> HHHHHHHSSENLYFQGHMRKIRVGLIFGGKSAEHEVSLQSARNILDALDPQRFEPVLIGIDKQGQWHVNDPDSFLLHADDPARIALHRSGRGVALLPGAQQQQLRPIQPEQALAQIDVVFPIVHGTLGEDGSLQGLLRMANLPFVGSGVLGSAVAMDKDMAKRVLRDARLAVAPFVCFDRHTAAHADVDTLIAQLGLPLFVKPANQGSSVGVSQVRTADAFAAALALALAYDHKVLVEAAVAGREIECAVLGNAVPHASVCGEVVVHDAFYSYATKYISEHGAEIVIPADIDAQ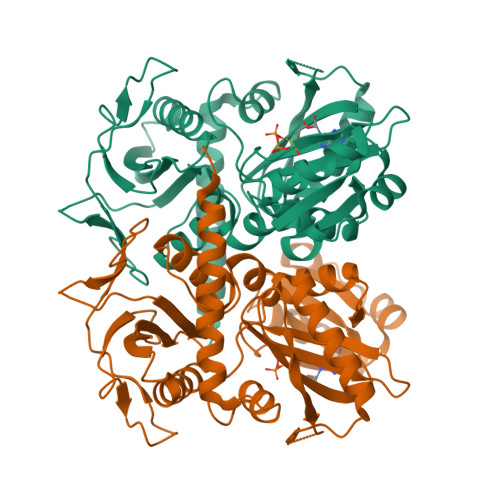TQQRIQQIAVQAYQALGCAGMARVDVFLCADGRIVINEVNTLPGFTRISVYPKLWQASGLDYRGLITRLIELALERHTDDQLLRSAVELH>[2x]GSWSVKELEDKNEELLSEIAHLKNEVARLKKLLQRCLAANQELRDAIRQSNQILRERAEELLHFQASQREEKEFLMSKFQEARKLVERLGLEKLELEDKNEELLSEIAHLKNEVARLKKLVGER

Inhibition of the protein-protein interaction between NEMO and IKKβ represents an attractive alternative strategy due to the crucial role of NEMO and its selective involvement in the canonical NF-κB pathway. We have previously reported the design and characterization of a coiled-coil stabilized NEMO construct encompassing the IKKβ-binding region fused to two ideal dimeric coiled-coil adaptors, at the N and C-terminus. Here we report the structure of the unliganded N-terminal domain of NEMO, utilizing the coiled-coil stabilized NEMO construct modified by four additional point mutations, designed to improve solution behavior and crystal packing. The crystal structure reveals that NEMO folds in an irregular dimeric coiled coil in the absence of IKKβ, with discontinuities in the heptad repeats causing an underwinding of the supercoil in the ligand binding region.

Mutations E56A and E57A, suggested by the Surface Entropy Reduction Server SERp29, were chosen to promote crystal lattice contacts between NEMO dimers, and as unlikely to affect IKKβ binding affinity (NEMO-EEAA). NEMO-EEAA is a homo-dimeric, irregular, parallel coiled coil of ∼175 Å in length. The regular coiled coil extends to the first two heptads of the NEMO sequence, to residue Ile65, and resumes after Phe97, encompassing the last 15 residues of the NEMO sequence and the C-terminal GCN4 adaptor. The interhelical spacing goes from an average value of 7.6 Å in the regular coiled-coil structure to a maximum of 11.5 Å for the stutter “heptad”. The most notable characteristic of the structure of NEMO (51–112) in the unbound form is a more compact packing of the two helices in the dimer, compared to the IKKβ bound structure, with an interhelical spacing reduced by up to 2.2 Å. The helix axis in the apo structure, between Lys90′ and Val104′, rotates towards the center of the bundle by about 35 degrees. Consequently, several of the side chains now occupy the IKKβ binding pocket. Analysis of normalized B-factors within the NEMO-EEAA structure shows increased values in residues 65–92 of chain B versus the remaining residues of the chain (all positive values, i.e. larger B-factor than average). The only accessible pocket in the unbound conformation of NEMO is pocket II, which represents the point of maximum opening of the bun and where CASTp locates a pocket involving the same residues contacting the ligand in the bound form.>GPGSHLAHPNLDTFTPEELLQQMKELLTENHQLKEAMKLNNQAMKGRFEELSAWTEKQKEERQFFEIQSKEAKERLMALSHE[2x];>GPGSYPSSNTLVEMTLGMKKLKEEMEGVVKELAENNHILERFGSLTMDGGLRNVDCL[2x]

OPTN is an ubiquitin-binding autophagy receptor, which is initially found to participate in the xenophagy and aggrephagy processes, and more recently is also demonstrated to involve in the PARKIN-dependent mitophagy. The N-terminal coiled-coil region of OPTN is responsible for its interaction with TANK-binding kinase 1 (TBK1), which is a noncanonical IκB kinase family member involved in innate immunity and autophagy. Here we biochemically and structurally characterize the interaction between OPTN and TBK1, and demonstrate that the direct association of OPTN N-terminal coiled-coil domain (NTD) with TBK1 CTD domain is responsible for the OPTN/TBK1 complex formation. The structures of OPTN NTD in complex with TBK1 CTD and the related NAP1/TBK1 complex solved in this study not only elucidate the detailed molecular mechanism underlying the OPTN and TBK1 interaction but also uncover a general interaction mode governing TBK1's binding to all of its currently identified binding adaptor proteins.

Fortunately, using this short OPTN fragment in complex with TBK1 CTD, we obtained high-quality crystals that diffracted to 2.05 Å resolution. In the final refined structural model, each asymmetric unit contains one OPTN(26–103)/TBK1 CTD complex molecule, which has a 2:2 stoichiometry and forms a symmetrical hetero-tetramer consisting of a OPTN dimer and two TBK1 CTD molecules. The OPTN(26–103)/TBK1 CTD complex adopts an overall elongated and atypical parallel four-helix bundle architecture. In the complex structure, the two OPTN molecules mainly form two crescent-shaped continuous α-helices with their C-terminal parts (residues 73–102) directly packing with each other to form a homo-dimeric interface and N-terminal parts head-to-head bridging across two TBK1 CTD molecules, each of which also adopts an α-helical configuration. Notably, the extreme C-terminal 11 amino acids (residues 719–729) of TBK1 CTD could not be traced in the complex structure, presumably due to the dynamic nature of this region. The binding interface between OPTN and TBK1 is within the N-terminal four-helix bundle core, whose interior is formed by 10 layers of interacting amino-acid side chains. Detailed structural analyses revealed that the assemblies of the 10 layers are mainly mediated by hydrophobic and polar interactions. In the complex structure, the C-terminal coiled-coil region (residues 73–102) of OPTN consists of four heptad repeats, and is responsible for the OPTN dimer formation. In the OPTN(26–103)/TBK1 CTD complex structure, the OPTN E50 residue is exposed to the solvent and plays an adjuvant role for the OPTN/TBK1 interaction by forming a charge–charge interaction with the positively charged TBK1 K694 residue, which is further neutralized by two nearby negatively charged OPTN E46 and TBK1 E698 residues.> GAMTIGRAKVYATLSKIFYHLFYDEAIPKDCREIIEKFGEIDFNLRSVLVRELRGSVLIKDMPQSLAEVYESVMKDFYERYGFQASELHADHIAVELAFMSKLV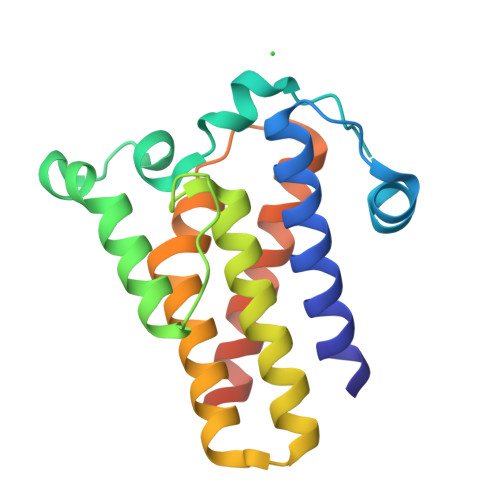EREISLAQQMKEEELYKIRAAQHRFIKAHLQPLVKNLPSAPLLNFVRDFVREDAKYLYSSLVGEKNEGADNN>MSAQTGTDLFKIADLFAYQVFDSRGFPTVACVVKLASGHTGEAMVPSGASTGEKEAIELRDGDPKAYFGKGVSQAVQNVNQTIAPKLIGLNATDQAAIDALMIQLDGTPNKAKLGANAILAVSLAVAKAAASAQKTSLFKYLANQVMGLNKTEFILTVPMLNVINGGAHADNNIDFQEFMIMPLGANSMHQALKMASETFHALQKLLKQRGLNTNKGDEGGFAPNLKLAEEALDLMVEAIKAAGYQPGSDIAIALDVAASEFYDDTTKRYVFKKG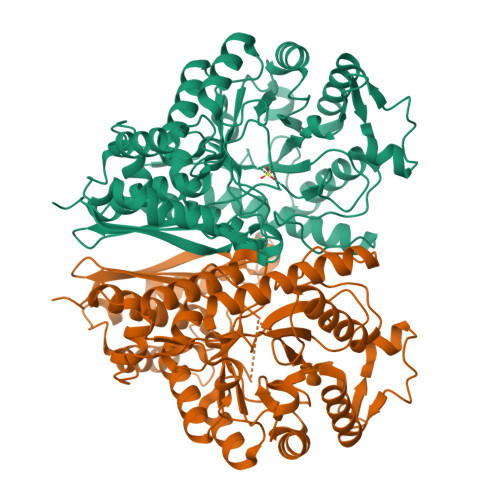IKAKILDEKEWSLTTAQMIAYLKKLTEQYPIISIEDGLSEHDWEGMETLTKTLGQHIQIVGDDLYCTNPAIAEKGVAHKATNSILIKLNQIGTLTETIKAINIAKDANWSQVISHRSGETEDTTIADLAVAACTGQIKTGSMSRSERIAKYNRLLQIELELGNNAKYLGWNTFKNIKPQKALEHHHHHH[4x]N-[(furan-3-yl)methyl]pyrrolidine-1-carboxamide | C10 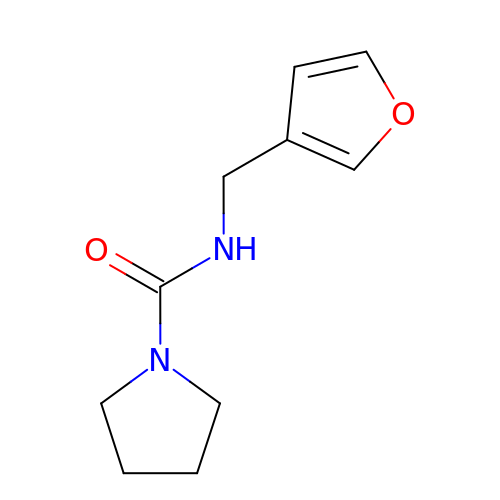H14 N2 O2 | ONGBBTQZWYAQQB-UHFFFAOYSA-N>[2x]GSALEKVPVEEYLVHALQGSVSSGQAHSLASLAKTWSSGSAKLQRLGPETEDNEGVLLTEKLKPVDYEYREEVHWMTHQPRVGRGSFGEVHRMKDKQTGFQCAVKKVRLEVFRVEELVACAGLSSPRIVPLYGAVREGPWVNIFMELLEGGSLGQLIKQMGCLPED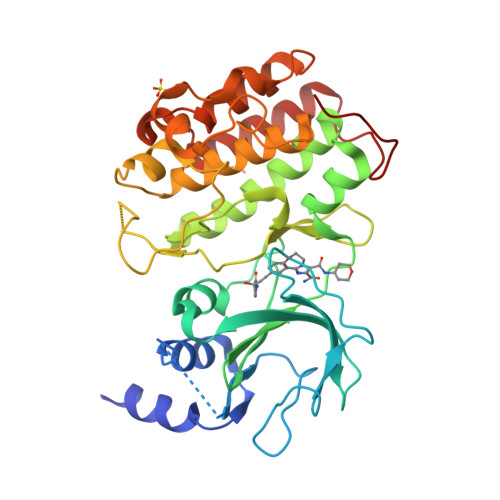RALYYLGQALEGLEYLHTRRILHGDVKADNVLLSSDGSRAALCDFGHALCLQPDGLGKSLLTGDYIPGTETHMAPEVVMGKPCDAKVDIWSSCCMMLHMLNGCHPWTQYFRGPLCLKIASEPPPIREIPPSCAPLTAQAIQEGLRKEPVHRASAMELRRKVGKALQEVGGLKSPWKGEYKEPR>MLEADDQGCIEEQGVEDSANEDSVDAKPDRSSFVPSLFSKKKKNVTMRSIKTTRDRVPTYQYNMNFEKLGKCIIINNKNFDKVTGMGVRNGTDKDAEALFKCFRSLGFDVIVYNDC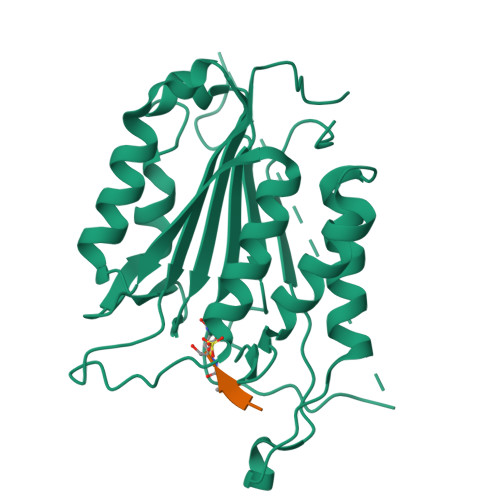SCAKMQDLLKKASEEDHTNAACFACILLSHGEENVIYGKDGVTPIKDLTAHFRGDRSKTLLEKPKLFFIQACRGTELDDGIQADSGPINDTDANPRYKIPVEADFLFAYSTVPGYYSWRSPGRGSWFVQALCSILEEHGKDLEIMQILTRVNDRVARHFESQSDDPHFHEKKQIPCVVSMLTKELYFSQ[2x]>MVVNMFEDIDTFEEAFNKLLREVLEFDLQNPFKDAKKVLCIEPHPDDCVIGMGGTIKKLSDMGVEVIYVCMTDGYMGTTDESLSGHELAAIRRKEEEESARLLGVKKIYWLNYRDTELPYSREVRKDLTKILRKEQPDGVFAPDPWLPYESHPDHRRTGFLAIESVAFSQLPNFSNT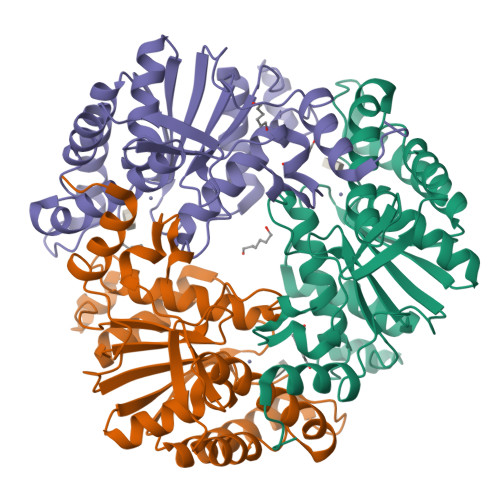DLDIGLNPYNSGSFIALYYTHKPNYIVDITDLMELKLKAIRVHRSQFPDDIWEKWEPFLRTIAMFYGEKIGVRYGEGFRIMPGLFYHITPFTDLI[3x]> MDKDEAWKQVEQLRREGATQIAYRSDDWRDLKEAWKKGADILIVDATDKDEAWKQVEQLRREGATQIAYRSDDWRDLKEAWKKGADILIVSEEMARHAPKDEAWKQVEQLRREGATQIAYRSDDWRDLKEAWKKGADILIVDATDKDEAWKQVEQLRREGATQIAYRSDDWRDLKEAWKKGADILIVDATGLEHHHHHH

The fold is composed of an eightfold repeat of βα‐units, with eight parallel β‐strands forming a circular sheet in the core that is surrounded by the eight α‐helices. The design called sTIM11 is a monomeric and stable protein that with its X‐ray structure provides a suitable starting point for further enzyme design approaches. With its compact structure it does however lack an extended surface or pocket as usually found in enzymes. Here we took steps towards the goal of diversifying de novo TIM barrel by extending sTIM11 by a simple structural element, namely an additional helix that we inserted in a loop at the upper part of the barrel.

Since the two halves of sTIM11 can assemble into a TIM‐barrel like dimer, we believed the loop in the middle of the protein sequence to be maximal tolerant for the structural modification and chose it as the target site for the helical extension. We further introduced a small change to the sTIM11 scaffold by removing two cysteine residues that were originally introduced to form a disulfide bridge to improve barrel closure. Moreover, the design showed a similar thermal stability to sTIM11noCys with a melting temperature of 66°C. The protein was crystallized and diffraction data collected and processed to a resolution of 1.58 Å. The introduced helix showed elevated B‐factors, making it more difficult to model. While a helical structure was formed, it is wound slightly different than expected and forms a 310 helix instead of a classical α‐helix. In addition, its position is slightly twisted and it packs more closely and flat onto the barrel surface compared to the design model, which projected the helix to be more exposed. Interestingly, the experimental structure revealed a different hydrophobic packing and showed Met94 to rather enter the barrel by inserting its side chain in between the β‐sheet core and the outer barrel α‐helix. Due to this, several polar contacts that had been predicted between the first residues of the inserted helix and its surrounding could not form, but a polar contact between Ser90 and Asp71 is established instead. Thus, the de novo TIM barrel accommodates the newly inserted 310 helix by a rearrangement of the packing of the barrel helix.HEXADECANE-1-SULFINIC ACID | 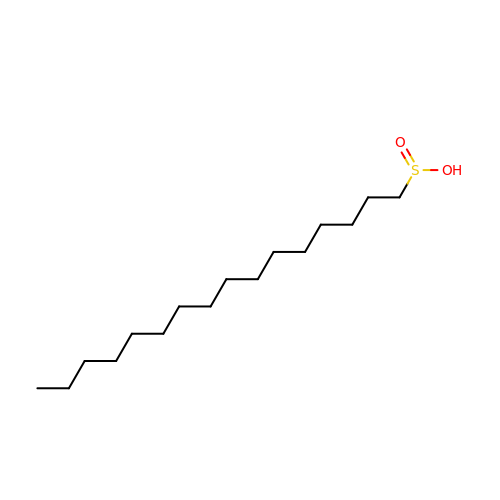C16 H34 O2 S | HBTBNXFVJYRYGI-UHFFFAOYSA-N> KVEEILEKALELVIPDEEEVRKGREAEEELRRRLDELGVEYVFVGSYARNTWLKGSLEIDVFLLFPEEFSKEELRERGLEIGKAVLDSYEIRYAEHPYVHGVVKGVEVDVVPCYKLKEPKNIKSAVDRTPFHHKWLEGRIKGKENEVRLLKGFLKANGIYGAEYKVR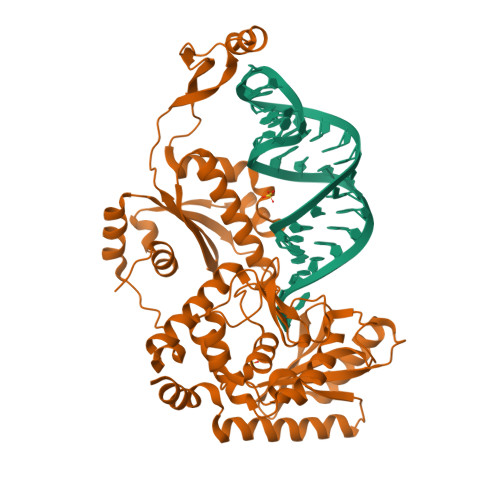GFSGYLCELLIVFYGSFLETVKNARRWTRRTVIDVAKGEVRKGEEFFVVDPVDEKRNVAANLSLDNLARFVHLCREFMEAPSLGFFKPKHPLEIEPERLRKIVEERGTAVFAVKFRKPDIVDDNLYPQLERASRKIFEFLERENFMPLRSAFKASEEFCYLLFECQIKEISRVFRRMGPQFEDERNVKKFLSRNRAFRPFIENGRWWAFEMRKFTTPEEGVRSYASTHWHTLGKNVGESIREYFEIISGEKLFKEPVTAELCEMMGVKD> SNPCAKPHGKKLATVKQIAQYYKRKAYIQLNERGSRSALKGDASQGQYDRGGKADDFKTKLCEINEKHSNARSNSLNPCNGKDNNKVRFNVGTPWQSGEKIATATDVYLPPRRQHFCTSNLEYLING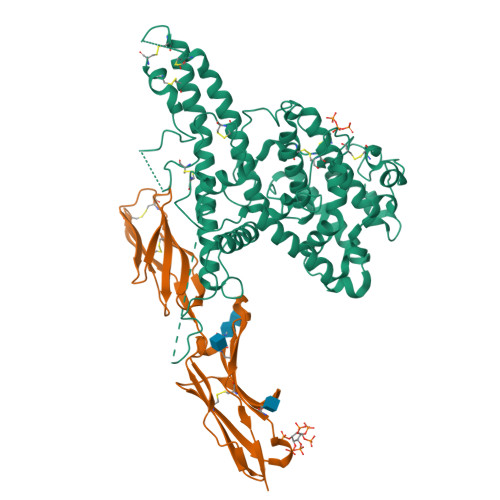GHQAILNVKNGKINHSFLGDVLLAAKYQAQHTMKDYKSKNDKEGICRAIRYSFADIGDIIKGTDLWDKDGGEIKTQNHLVTIFDKIKAQLPKDIKGKYTGTKHLELRKDWWEANRDQVWKAMQCGNDNPCSGESDHTPLHDYIPQRLRWMTEWAEWYCKEQSRLYDKLKVCEECMRKGESCTKGSGECATCKEACEEYNKEIKKWEQQWDAISYKYLMLYAKARITAINGGPGYYNTEVQEEDKPVVDFLYNLYLQNGGKKGPPPDTHRVKALIARVKRDAARNRVKRADGSSATRVTATTTITPYSTAAGYIHQEAHIGDCQKQTQFCKNKNGSDVSDTEADPTYAFRDKPHDHDTACKC;> QTSVSPSKVILPRGGSVLVTCSTSCDQPKLLGIETPLPKKELLLPGNNRKVYELSNVQEDSQPMCYSNCPDGQSTAKTFLTVYWTPERVELAPLPSWQPVGKNLTLRCQVEGGAPRANLTVVLLRGEKELKREPAVGEPAEVTTTVLVRRDHHGANFSCRTELDLRPQGLELFENTSAPYQLQTFG> GSPGISGGGGGILDSMAEIVADKTVEVVKNAIETADGALDLYN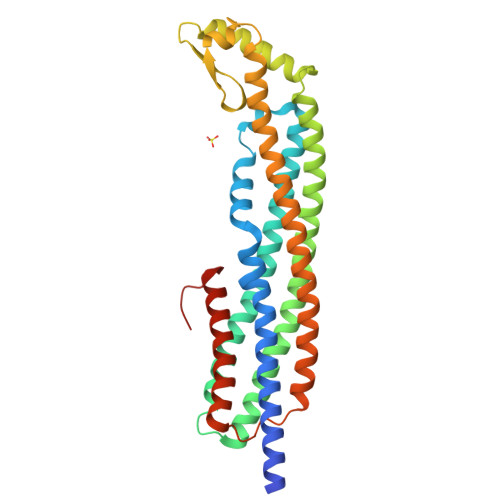KYLDQVIPWQTFDETIKELSRFKQEYSQAASVLVGDIKTLLMDSQDKYFEATQTVYEWCGVATQLLAAYILLFDEYNEKKASAQKDILIKVLDDGITKLNEAQKSLLVSSQSFNNASGKLLALDSQLTNDFSEKSSYFQSQVDKIRKEAYAGAAAGVVVGPFGLIISYSIAAGVVEGKLIPELKNKLKSVQNFFTTLSNTVKQANKDIDAAKLKLTTEIAAIGEIKTETETTRFYVDYDDLMLSLLKEAAKKMINTCNEYQKRHGKKTLFEVPEV>MAPAKSPRAWQRMLSGRRLDLLDPSPLDVEIADIAHGLARVARWNGQTRGDHAFTVAQHCLIVETIFCRMCPGATPDEMQMALLHDAPEYVIGDMISPFKSVVGGGYKTVEKRLEAAVHLRFGLPPHASRELKDRIKKADTVAAF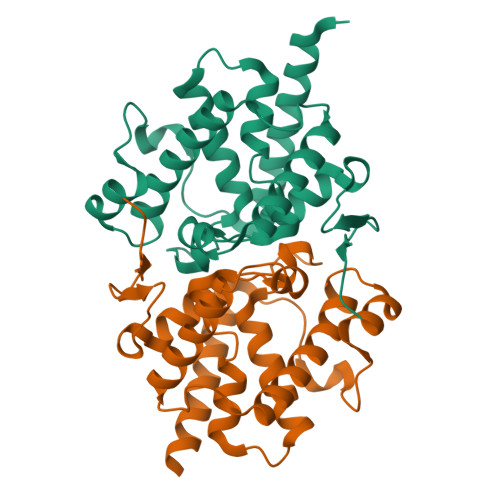FEATELAGFSTAEAQKFFGLPRGITRDMFDIIPLPSTEAQRLFIARFEAIETLRVTRTGGAV[4x]>[4x]VLGGHECQPHSQPWQAALFQGQQLLCGGVLVGGNWVLTAAHCKKPKYTVRLGDHSLQNKDGPEQEIPVVQSIPHPCYNSSDVEDHNHDLMLLQLRDQASLGSKVKPISLADHCTQPGQKCTVSGWGTVTSPRENFPDTLNCAEVKIFPQKKCEDAYPGQITDGMVCAGSSKGADTCQGDSGGPLVCDGALQGITSWGSDPCGRSDKPGVYTNICRYLDWIKKIIGSKG

KLK8, formerly termed hK8, belongs to the 15 human kallikrein-related peptidases of the trypsin-like family S1A, with the MEROPS code S01.2445. KLK8 is secreted as an inactive pro-enzyme, whereby a signal peptide is cut off, followed by propeptide cleavage at the Lys15-Val16 bond, releasing active enzyme. As in most trypsin-like serine proteinases the KLK8 chain consists of two six-stranded β-barrels that can be considered as half-domains. At their interface the catalytic triad of Ser195, His57 and Asp102 is situated above the specificity subsites S4 to S4′, aligned from left to right in the standard orientation.

Upon soaking the crystals with ZnCl2, one cell constant approximately doubled in length, accompanied by a transition to space group P21, with four molecules per asymmetric unit. The corresponding 2.1 Å structure of KLK8, in which Zn2+ was not clearly identified, is referred to as KLK8-leup and resembles largely the KLK8-Ca molecule. By contrast, the P21 form of KLK8-leup contains four copies of the aldehyde inhibitor leupeptin, with the sequence acetyl-Leu1i-Leu2i-Argininal3i. Leupeptin binds covalently to Ser195 as analogue of an acyl intermediate in the canonical conformation. The P1-Arg3i aldehyde group in KLK8-leup is covalently linked to Ser195 Oγ as hemiacetal, with the oxygen occupying the oxyanion hole in the four KLK8 copies. Similar to a substrate, leupeptin forms a short antiparallel β-sheet with two backbone hydrogen bonds between P3-Leu1i and Gly216, and the amide of P1-Arg3i and the carbonyl oxygen of Ser214. The Arg3i side chain is buried in the S1 specificity pocket, which is rather hydrophobic in the upper region, whereas at the bottom the side-chains of Thr190, Ser217, Tyr228, and a water molecule bound to the Ser217 carbonyl O contribute to a polar environment. The negatively charged carboxylate of Asp189 forms a tight salt bridge to the positively charged Arg3i guanidyl group. The funnel-shaped S2 subsite of KLK8 is bordered by the hydrophobic side-chains of His57, His99, and partially Trp215, which explains very well the accommodation of the Leu2i side-chain of the inhibitor and the preference for the aliphatic Val and Leu residues in the substrate profiling. Also, the specific interactions of the P4 to P1 residues can be well explained on a structural level by the complex of KLK8 with the leupeptin inhibitor.> STNKVNKERTFLAVKPDGVARGLVGEIIARYEKKGFVLVGLKQLVPTKDLAESHYAEHKERPFFGGLVSFITSGPVVAMVFEGKGVVASARLMIGVTNPLASAPGSIRGDFGVDVGRNIIHGSDSVESANREIALWFKPEELLTEVKPN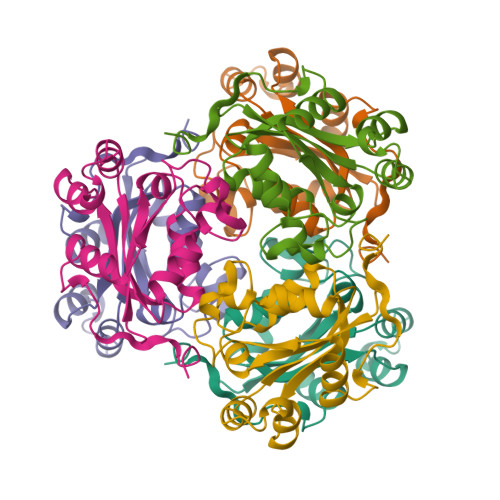PNLYE>[2x]SNAMKTRLNKTSLNQALLPTSTAGSLPKPLWLAEPETLWSPWKLQGEELITGKHDALRLSLQDQQLAGIDIVSDGEQTRQHFVTTFIEHLNGVDFSKRKIVKIRDRYDASVPTVVGPVSRQKSVFVEDAKFLRKQTTQPIKWALPGPMTMIDTLYDDHYKSREKLAWEFAKILNEEAKELEAAGVDIIQFDEPAFNVFFDEVNDWGIACLERAIEGLKCETAVHICYGYGIKANTDWKKTLG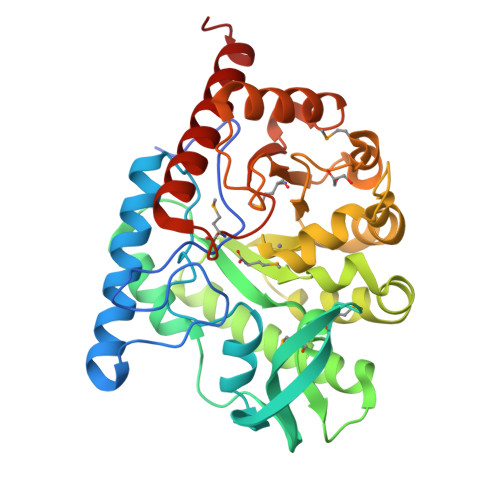SEWRQYEEVFPKLQKSNIDIISLECHNSHVPMELLELIRGKKVMVGAIDVATDTIETAEEVADTLRKALKFVDADKLYPCTNCGMTPLSHQVTRGKLNALSAGAEIVRKELLALR> MSVDSSGMEPPPLPSDGPE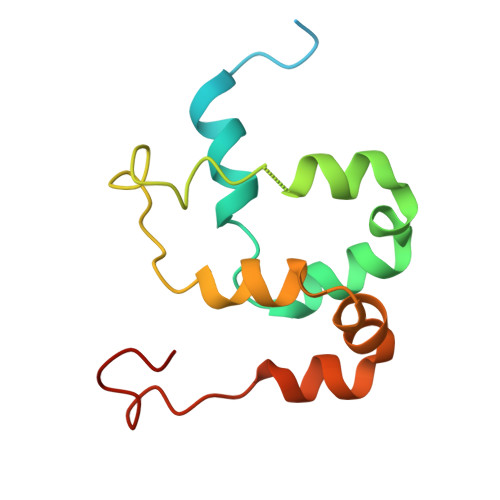EPKHGGHTRFELELEFVQALSNPEYVNWLASRKYLMNPAFVAYLDYLQYWSRPPYLKYLTYPTATLRMLQLLQSERFRQEILVPDVAWQLRLEGMKAAVLWHKEG3-AMINO-3-OXOPROPANOIC 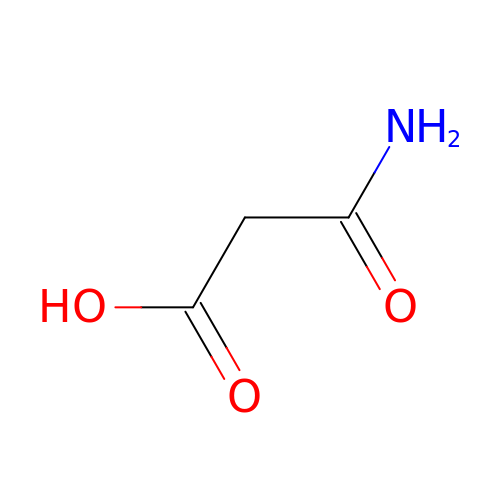ACID | C3 H5 N O3 | CGJMROBVSBIBKP-UHFFFAOYSA-N>[4x]HHHHHHDLVEEVDWKDIPVPADAGPNMKWEFQEISDNFEYEAPADNKGSEFLEKWDDFYHNAWAGPGLTEW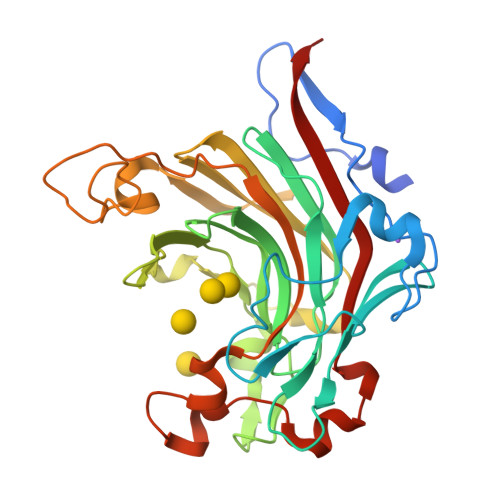KRDRSYVADGELKMWATRKPGSDKINMGCITSKTRVVYPVYIEARAKVMNSTLASDVWLLSADDTQEIDILDAYGADYSESAGKDHSYFSKKVHISHHVFIRDPFQDYQPKDAGSWFEDGTVWNKEFHRFGVYWRDPWHLEYYIDGVLVRTVSGKDIIDPKHFTNTTDPGNTEIDTRTGLNKEMDIIINTEDQTWRSSPASGLQSNTYTPTDNELSNIENNTFGVDWIRIYKPVEKL>MDGGMWLMQQINGQVARMKSLGMQLEAADIYNPNGSSLKDAVVMFDGGCTGVLVSNQGLLLTNHHCGYDQIQKHSSVQHNYLKDGFWSYSLAEELVNPGLEVEIVDEITDVTAAVKKELERIKKPSGLEFLSPRYLSSLAPEIVGKKAASRPGYRYEIKAFYGGNRYYMFTKKVFRDVRLVAAPPSSIGKFGSDTDNWAWPRHTGDFSIFRLYADKNGNPAEYSKDNVPYRPKRWVKVNAQGVKEGDFALIMGYPGTTYKFFTADEVTEWSEIDNNIRIEMRGILQDVMLREMLADPKINIMYAAKYASSQNGYKRAQGANWAIRRRSLREIKLAQQQEVLAWAKQKGIATTEEAVRAISKAIEGRQDLRMRQRYLLEGILMGIEMSNAPAADSDIADHWDDPARREAGLQSIRKQFEAFFNKDYSPEVEKDQLAIALLTRYAERIPAEKQPISIREGIAEYGSAKAYVEMIFDKSIYASRERFEEFMKNPDRDRLLRDPMSRFAASVAYEHQKLAKEVAAFDAPLAAAQRSYVASVLDMKGQPNLAPDANLTLRFTYGEIKGYQPRDVVTYGAKSTLEGVMEKEDPNNWEYVVDPKLKALYEAKNYGRYANSDGSMPVNFCATTHTTGGNAGSPVMNARGELIGLNFDRNWEGVGGDIEYLPNYQRSIILDIRYLLFIIDKFAGCQRLIDEIQPQFHHHHHH[2x]

Here, we show that dipeptidyl peptidase 11 (DPP11), a central metabolic enzyme in these bacteria, undergoes a conformational change upon peptide binding to distinguish substrates from end products. As previously reported, the overall fold of DPP11 comprises a bilobal architecture. The upper helical domain dictates the specificity of the enzyme and caps the catalytic domain, which has a typical chymotrypsin double β-barrel fold. The active site of DPP11 lays in a wide cleft running through the middle of the protein between the catalytic and helical domains, which contributes to the formation of the substrate binding subsites.

We determined the structures for the inactive constructs PgDPP1122-720 S655A, PeDPP1122-717 S652A and its complexes with the dipeptides Arg-Asp and Arg-Glu, as well as the substrate Leu-Asp-Val-Trp, at 2.4, 2.85, 2.2, 2.1 and 2.6 Å resolution, referred to as PgDPP11, PeDPP11, PeDPP11:RD, PeDPP11:RE and PeDPP11:LDVWs, respectively. A notable difference between the unbound PeDPP11 and its complexes with peptides is the conformational change bringing the helical and catalytic domains closer. This movement yields an approximate rotation of 22° of one domain relative to the other with a negligible translational component. The bound-peptide is anchored at its N-terminus primarily by N332 (N-anchor) located in the helical domain. The distance between the N-anchor and the catalytic S652 permits accommodation of only two amino acid residues, revealing how the enzyme acquires its dipeptidyl peptidase specificity. Evolutionary conserved R670 is responsible for the Asp/Glu specificity at subsite S1: its guanidinium group directly interacts with the substrate carboxyl group of Asp/Glu. Analysis of PeDPP11:RD using Naccess32 revealed a large loss of solvent-accessible area upon peptide binding, approximately 1430 Å2. However, our crystal structures of DPP11 in complex with LDVW and dipeptide RD are both in closed conformation, excluding the possibility that solvent released from the protein’s cleft would explain the larger increase in entropy upon substrate binding.>MTSCHIAEEHIQKVAIFGGTHGNELTGVFLVKHWLENGAEIQRTGLEVKPFITNPRAVKKCTRYIDCDLNRIFDLENLGKKMSEDLPYEVRRAQEINHLFGPKDSEDSYDIIFDLHNTTSNMGCTLILEDSRNNFLIQMFHYIKTSLAPLPCYVYLIEHPSLKYATTRSIAKYPVGIEVGPQPQGVLRADILDQMRKMIKHALDFIHHFNEGKEFPPCAIEVYKIIEKVDYPRDENGEIAAII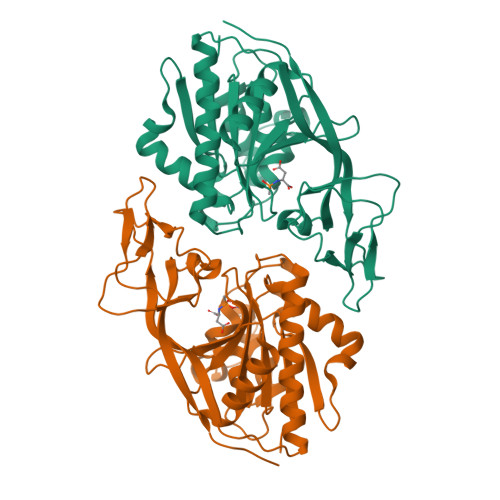HPNLQDQDWKPLHPGDPMFLTLDGKTIPLGGDCTVYPVFVNAAAYYEKKEAFAKTTKLTLNAKSIRCCLH[2x]>[3x]MHLKIVCLSDEVREMYKNHKTHHEGDSGLDLFIVKDEVLKPKSTTFVKLGIKAIALQYKSNYYYKCEKSENKKKDDDKSNIVNTSFLLFPRSSI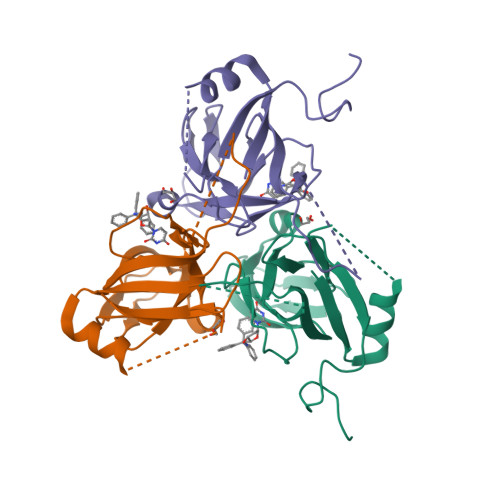SKTPLRLANSIGLIDAGYRGEIIAALDNTSDQEYHIKKNDKLVQLVSFTGEPLSFELVEELDETSRGEGGFGSTSNNKYLEHHHHHH> MLQRTTLRCYSALVGQATPVLLGSKGGTPKRKKNPMQLRRKTYGLHFKERYLKLEEWYFCPLCAEPKKQ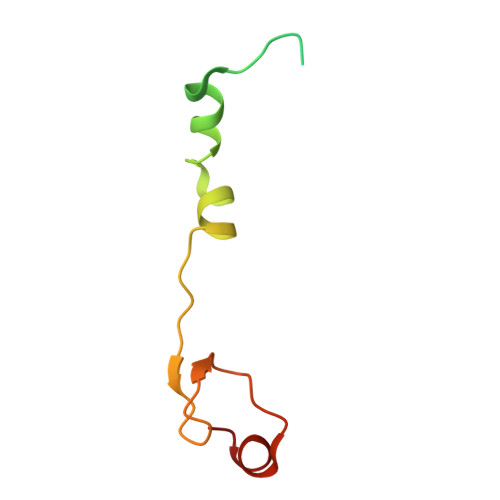GEWCRREDCRQIKP> KLLLEGVKEQDPVDKFTYLLLQPLTEATLSDAVNFIVEKYSAELPDEGDASLVVRSQLGCQFFFLVTRTLAHDQRELAKLVQTLIPRPVRLEVFPGLQRSVFKSSVFLGHHIIQIFMGAKKPFQDWSFVGLAQDFECPWRRLAIAELLKKFSVSVVEKVFDNPVALIPQHESDNEALIELVTNALRFALWIVEFYETETNEKSIKELAFLDHSSKTLLIESFTKFLQ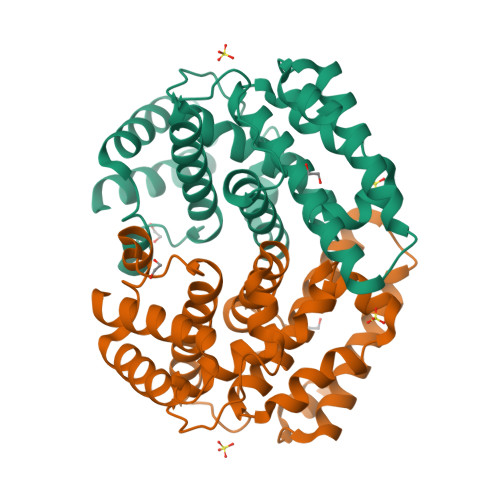GKDVKDQDHLKRIIDALEKS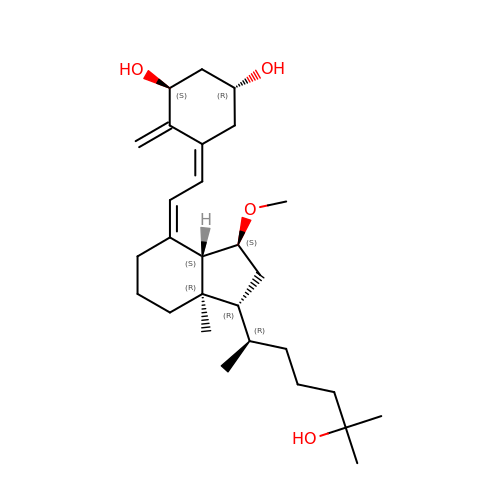(1R,3S,5Z)-5-[(2E)-2-[(1R,3S,3aS,7aR)-1-[(2R)-6-hydroxy-6-methyl-heptan-2-yl]-3-methoxy-7a-methyl-2,3,3a,5,6,7-hexahydro-1H-inden-4-ylidene]ethylidene]-4-methylidene-cyclohexane-1,3-diol | C28 H46 O4 | MKYCMLKYANTZFR-GSVKQXOCSA-N>[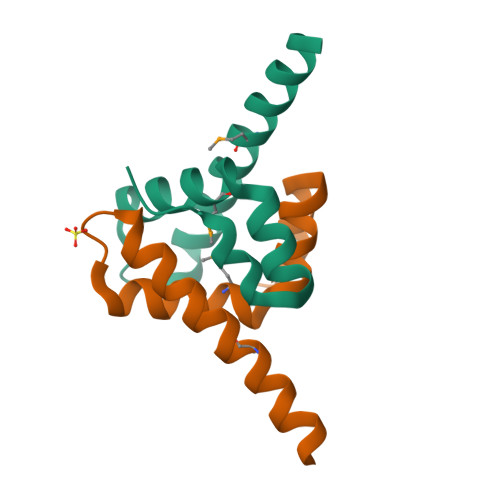5x]SNAMAVETLYRSTRDLETTFVDRKLADAHDQMLELAELLTDVLIKNVPGLSEKHAEDASIYMAKNRAVFAAAFKNNATALSELSEPAESEG>[8x]MGHHHHHHLVPRGSHKRPMDTEEAEELVRQWENVKAEALGPTHQVYSLSEVLDES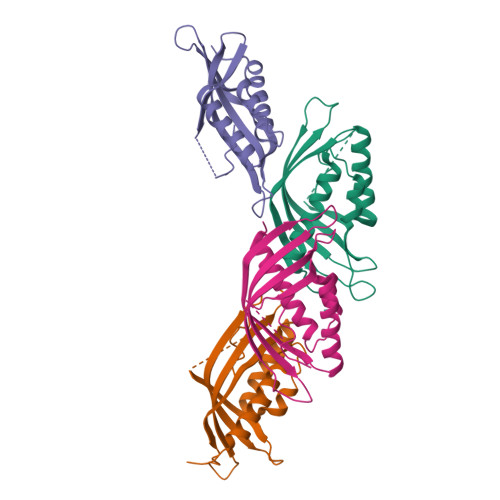MLVQWQTLAQTAEAKSCYWRFVLLHLEVLQAHIFEDGIAGEAAEIEALLEEAAELVDESQPKNAKYYSTYKIRYILKKQEDGLWKFCQSDIQIQKGSGSGSGSGSGSRKTYGRDKSSADRSLDHLDVMMARG> MLK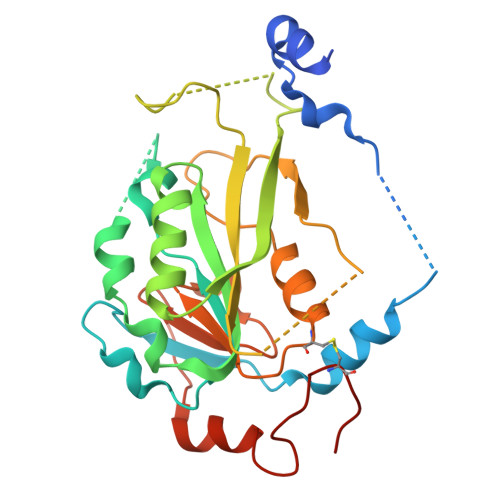GTQSLNPHNDYCQHFVDTGHRPQNFIRDVGLADRFEEYPKLRELIRLKDELIAKSNTPPMYLQADIEAFDIRELTPKFDVILLEPPLEEYYRETGITANEKCWTWDDIMKLEIDEIAAPRSFIFLWCGSGEGLDLGRVCLRKWGYRRCEDICWIKTNKNNPGKTKTLDPKAVFQRTKEHCLMGIKGTVKRSTDGDFIHANVDIDLIITEEPEIGNIEKPVEIFHIIEHFCLGRRRLHLFGRDSTIRPGWLTVGPTLTNSNYNAETYASYFSAPNSYLTGCTEEIERL>[2x]MVSGFAMPKIWRKLAMDIPVNAAKPGRRRYLTLVMIFITVVICYVDRANLAVASAHIQEEFGITKAEMGYVFSAFAWLYTLCQIPGGWFLDRVGSRVTYFIAIFGWSVATLFQGFATGLMSLIGLRAITGIFQAPAFPTNNRMVTSWFPEHERASAVGFYTSGQFVGLAFLTPLLIWIQEMLSWHWVFIVTGGIGIIWSLIWFKVYQPPRLTKGISKAELDYIRDGGGLVDGDAPVKKEARQPLTAKDWKLVFHRKLIGVYLGQFAVASTLWFFLTWFPNYLTQEKGITALKAGFMTTVPFLAAFVGVLLSGWVADLLVRKGFSLGFARKTPIICGLLISTCIMGANYTNDPMMIMCLMALAFFGNGFASITWSLVSSLAPMRLIGLTGGVFNFAGGLGGITVPLVVGYLAQGYGFAPALVYISAVALIGALSYILLVGDVKRVGSLVPRGSGSHHHHHH

Members of the solute carrier 17 (SLC17) family catalyze the coupled transport of anions driven by a proton electrochemical gradient ΔμH+ (= Δψ − 2.3× (RT/F) × ΔpH, where R is the gas constant, T is temperature, and F is Faraday’s constant), with contributions from both electrical potential Δψ and proton gradient ΔpH (pHo/pHi). The D-galactonate transporter (DgoT) gene lies within an operon devoted to the metabolism of D-galactonate, suggesting a role in transport of this acidic sugar. DgoT is composed of 12 TM helices and belongs to the MFS fold. Two 6-helix bundles (N- and C-terminal domains) are related by a pseudo 2-fold symmetry axis perpendicular to the membrane plane.

We were able to crystallize E133Q DgoT with D-galactonate bound. At pH 9.0, this complex crystallized in an outward-facing conformation, in a different crystal form than for the WT protein alone, and refined to an R-factor/Rfree of 28.5%/30.0% at 3.5 Å resolution. As with the inward-open conformation, 2 essentially identical monomers (rmsd of 0.63 Å between their 345 Cα atoms) pack in pairs closely against each other sharing contacts from the lipophilic surface but in an antiparallel arrangement in the asymmetric unit (i.e., one molecule with its cytoplasmic side up packs against another with its cytoplasmic side down in a noncrystallographic 2-fold orientation). The structure includes residues 24 to 443 except for the 11–amino acid dynamic region in the cytoplasmic loop (residues 231–243) and 13–amino acid periplasmic end of TM7 (residues 276–291). In the outward-facing structure, Arg47 (TM1) forms a direct electrostatic interaction with the carboxyl group in D-galactonate through a 3.6 Å salt bridge. Four residues (Asn393, Gln264, serine-370 [Ser370], and Gln164) provide 8 hydrogen bonds with the 5 substrate −OH groups and confer high specificity. In addition to the rigid-body motions of N- and C-terminal lobes, TM7 bends inward over the substrate and provides a periplasmic gate for the outwardly oriented occluded state. Preventing access to the cytoplasmic side, TM4 and TM10 form major interhelical contacts in the outward-facing state. Aromatic residues Phe137 in TM4 and tryptophan-373 (Trp373) in TM10 both make hydrophobic interactions with the aliphatic surface of D-galactonate. In the outward-facing conformation, TM4 has a kink at Pro135, whereas TM10 is continuous.> MSLALLLGYELPLTGANAAYGRVFQEAARLQLDRFNAAGGV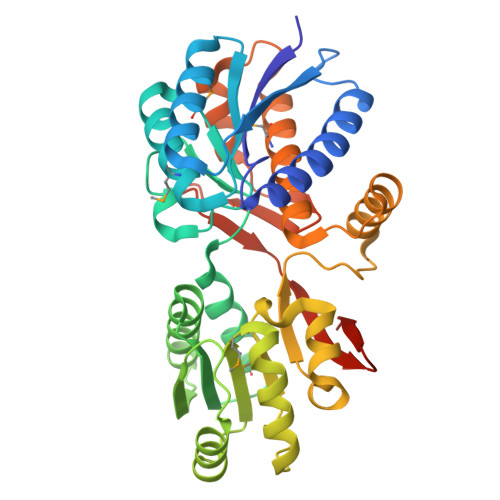GGRPVDILYADSRDDADQARTIARAFVDDPRVVGVLGDFSSTVSMAAGSIYGKEGMPQLSPTAAHPDYIKISPWQFRAITTPAFEGPNNAAWMIGDGFTSVAVIGVTTDWGLSSAQAFRKAFELRGGAVVVNEEVPPGNRRFDDVIDEIEDEAPQAIYLAMAYEDAAPFLRALRARGSALPVYGSSALYSPKFIDLGGPAVEGVRLATAFVLGASDPVVVEFVSAYETLYGAIPTLFAAHGYDAVGIMLAAVGRAGPEVTRESLRDALAATDRYAGVTGITRFDPETRETTKILTRLVVREGDFRVIDREGHHHHHH> MGSSFEVIARTAYEEGRTRLATELLNHEPRAGRQVPLLLSMEEDELALDKAIESGDTDLIYFVIHQLRRKLPLASFFRVVSSRPTASAMVEALARNSDGDGNEDTALLKDLYYQDDRRLDGASVFIREALQQPETRTASDKLDLAANLLQGNQKEHVFELGALKEAKMLLRMQETFERDLTDSFVGLSVNQTMFKLIKLGYHGRAKKIQSEFKVPE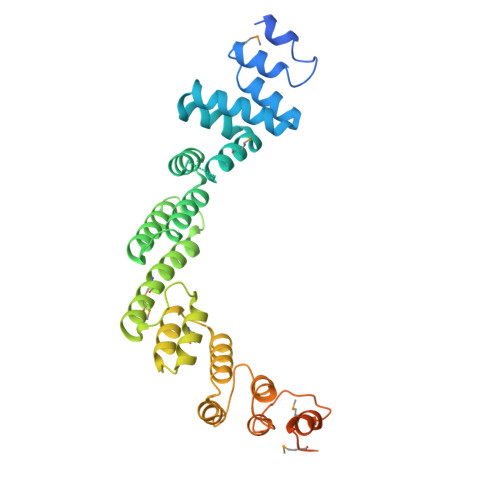RVAWWIRLQALVAKRDWNEIEEISRQRKSPIGWEPFFNQVLQAGNPRLAATFIPKCTNLEPGQTITMYEKCGMRVKAAEEAVRLKDTEAWNRLLEAAGRNTAEGREIERLGATVFKK> DLTVSLIPVS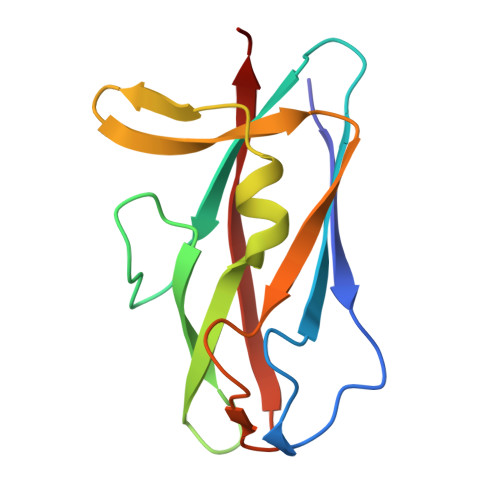GLKAGKNAPSAKIAKLVVNSTTLKEFGVRGISNNVVDSTGTAWRVAGKNTGKEIGVGLSSDSLRRSDSTEKWNGVNWMTFNSNDTLDIVLTGPAQNVTADTYPITLDVVGYQP>GSHMPGPVARLAPQAVLTPPSAASLFLVLVAGDSDDDRATVCDVISGIDGPLKAVGFRELAGSLSCVVGVGAQFWDRVSASSKPAHLHPFVPLSGPVHSAPSTPGDLLFHIKAARKDLCFELGRQIVSALGSAATVVDEVHGFRYFDSRDLLGFVDGTENPTDDDAADSALIGDEDPDFRGGSYVIVQKYLHDMSAWNTLSTEEQERVIGRTKLENVELDDDAQPSNSHVTLNTIVDDDGVEHDILRDAMAFGS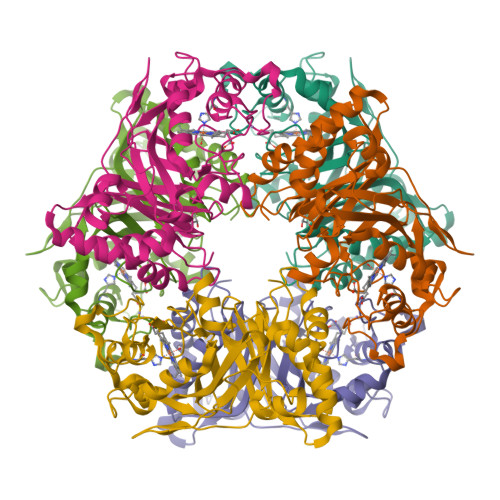LGEAEYGTYFIGYAKDPAVTELMLRRMFLGEPPGNYDRVLDFSTAATGTLFFVPSRDVLESLGDEPAGAESAPEDPVEPAAAGPYDLSLKIGGLKGVSQ[3x]> LPPKVSVFVPPRDGFFGNPRKSKLICQATGFSPRQIQVSWLREGKQVGSGVTTDQVQAEAKESGPTTYKVTSTLTIKESDWLGQSMFTCRVDHRGLTFQQNASSMCVPDQDTAIRVFAIPPSFASIFLTKSTKLTCLVTDLTTYDSVTISWTRQNGEAVKTHTNISESHPNATFSAVGEASICEDDWNSGERFTCTVTHTDLPSPLKQTISRPKGVALHRPDVYLLPPAREQLNLRESATI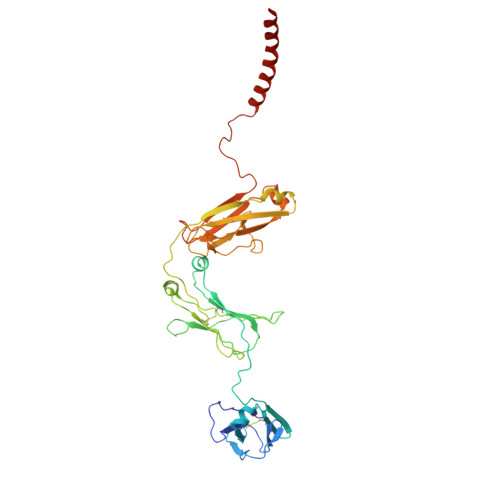TCLVTGFSPADVFVQWMQRGQPLSPEKYVTSAPMPEPQAPGRYFAHSILTVSEEEWNTGETYTCVVAHEALPNRVTERTVDKSTEGEVSADEEGFENLWATASTFIVLFLLSLFYSTTVTLFK> MKTSDANETEDHLESLICKVGEKSACSLESNLEGLAGVLEADLPNYKSKILRLLCTVARLLPEKLTIYTTLVGLLNARNYNFGGEFVEAMIRQLKESLKANNYNEAVYLVRFLSDLVNCHVIAAPSMVAMFENFVSVTQEEDVPQVRRDWYVYAFLSSLPWVGKELYEKKDAEMDRIFANTESYLKRRQKTHVPMLQVWTADKPHPQEEYLDCLWAQIQKLKKDRWQERHILRPYLAFDSILCEALQHNLPPFTPPPHTEDSVYPMPRVIFRMFDYTDDPEGPVMPGSHSVERFVIEENLHCIIKSHWKERKTCAAQLVSYPGKNKIPLNYHIVEVIFAELFQLPAPPHIDVMYTTLLIELCKLQPGSLPQV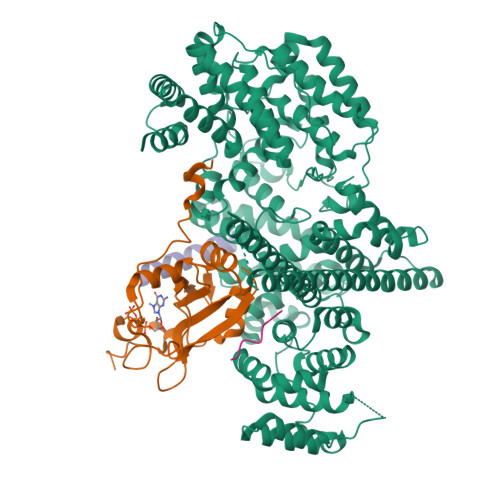LAQATEMLYMRLDTMNTTCVDRFINWFSHHLSNFQFRWSWEDWSDCLSQDPESPKPKFVREVLEKCMRLSYHQRILDIVPPTFSALCPANPTCIYKYGDESSNSLPGHSVALCLAVAFKSKATNDEIFSILKDVPNPNQDDDDDEGFSFNPLKIEVFVQTLLHLAAKSFSHSFSALAKFHEVFKTLAESDEGKLHVLRVMFEVWRNHPQMIAVLVDKMIRTQIVDCAAVANWIFSSELSRDFTRLFVWEILHSTIRKMNKHVLKIQKELEEAKEKLARQHKRRSDDDDRSSDRKDGVLEEQIERLQEKVESAQSEQKNLFLVIFQRFIMILTEHLVRCETDGTSVLTPWYKNCIERLQQIFLQHHQIIQQYMVTLENLLFTAELDPHILAVFQQFCALQA;> MSGGLLKALRSDSYVELSQYRDQHFRGDNEEQEKLLKKSCTLYVGNLSFYTTEEQIYELFSKSGDIKKIIMGLDKMKKTACGFCFVEYYSRADAENAMRYINGTRLDDRIIRTDWDAGFKEGRQYGRGRSGGQVRDEYRQDYDAGRGGYGKLAQNQ;>MALEVGDMEDGQLSDSDSDMTVAPSDRPLQLPKVLGGDSAMRAFQNTATACAPVSHYRAVESVDSSEESFSDSDDDSCLWKRKRQKCFNPPPKPEPFQFGQSSQKPPVAGGKKINNIWGAVLQEQNQDAVATELGILGMEGTIDRSRQSETYNYLLAKKLRKESQEHTKDLDKELDEYMHGGKKMGSKEEENGQGHLKRKRPVKDRLGNRPEMNYKGRYEITAEDSQEKVADEISFRLQEPKKDLIARVVRIIGNKKAIELLMETAEVEQNGGLFIMNGSRRRTPGGVFLNLLKNTPSISEEQIKDIFYIENQKEYENKKAARKRRTQVLGKKMKQAIKSLNFQEDDDTSRETFASDTNEALASLDESQEGHAEAKLEAEEAIEVDHSHDLDIF[2x]> MGRTVVVLGGGISGLAASYHLSRAPCPPKVVLVESSERLGGWIRSVRGPNGAIFELGPRGIRPAGALGARTLLLVSELGLDSEVLPVRGDHPAAQNRFLYVGGALHALPTGLRGLLRPSPPFSKPLFWAGLRELTKPRGKEPDETVHSFAQRRLGPEVASLAMDSLCRGVFAGNSRELSIRSCFPSLFQAEQTHRSILLGLLLGAGRTPQPDSALIRQALAERWSQWSLRGGLEMLPQALETHLTSRGVSVLRGQPV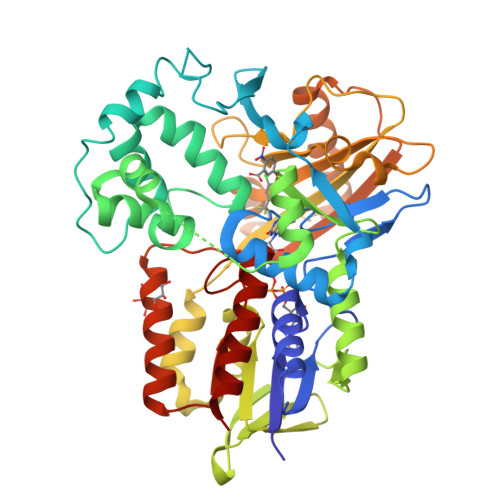CGLSLQAEGRWKVSLRDSSLEADHVISAIPASVLSELLPAEAAPLARALSAITAVSVAVVNLQYQGAHLPVQGFGHLVPSSEDPGVLGIVYDSVAFPEQDGSPPGLRVTVMLGGSWLQTLEASGCVLSQELFQQRAQEAAATQLGLKEMPSHCLVHLHKNCIPQYTLGHWQKLESARQFLTAHRLPLTLAGASYEGVAVNDCIESGRQAAVSVLGTEPNS> SYYHHHHHHLESTSLYKKAGLKIKAVGAYSAKQPLEPMDITRREPGPNDVKIEIAYCGVCHSDLHQVRSEWAGTVYPCVPGHEIVGRVVAVGDQVEKYAPGDLVGVGCIVDSCKHCEECEDGLENYCDHMTGTYNSPTPDEPGHTLGGYSQQIVVHERYVLRIRHPQEQLAAVAPLLCAGITTYSPLRHWQAGPGKKVGVVGIGGLGHMGIKLAHAMGAHVVAFTTSEAKREAAKALGADEVVNSRNADEMAAHLKSFDFILNTVAAPHNLDDFTTLLKRDGTMTLVGAPATPHKSPEVFNLIMKRRAIAGSMIGGIPETQEMLDFCA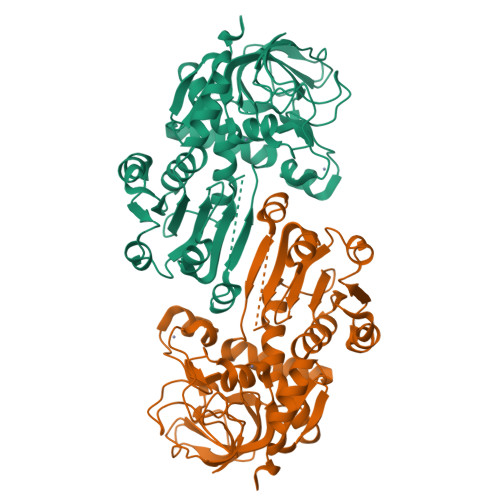EHGIVADIEMIRADQINEAYERMLRGDVKYRFVIDNRTLTD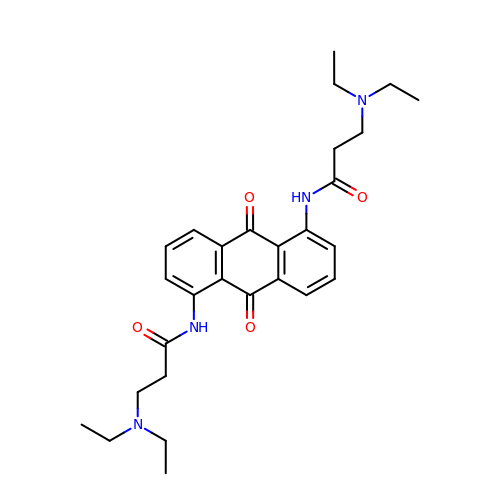1,5-BIS[3-(DIETHYLAMINO)PROPIONAMIDO]ANTHRACENE-9,10-DIONE | C28 H36 N4 O4 | VJLWMFJSEUYNRS-UHFFFAOYSA-N> GHMRQSTLHTRLSTGPGGSMRSSIEIFNIRTRKMRVVWQTPELFE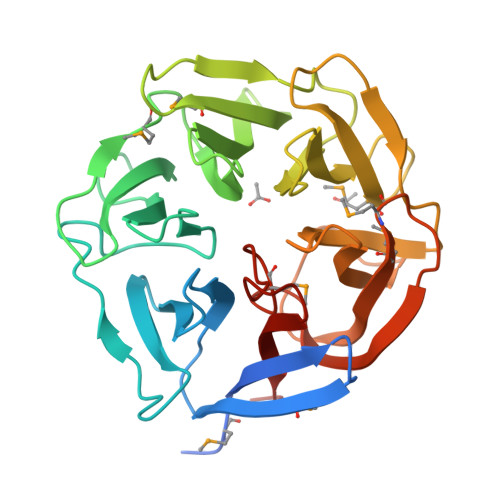APNWSPDGKYLLLNSEGLLYRLSLAGDPSPEKVDTGFATICNNDHGISPDGALYAISDKVEFGKSAIYLLPSTGGTPRLMTKNLPSYWHGWSPDGKSFTYCGIRDQVFDIYSMDIDSGVETRLTHGEGRNDGPDYSPDGRWIYFNSSRTGQMQIWRVRVDGSSVERITDSAYGDWFPHPSPSGDKVVFVSYDADVFDHPRDLDVRVQLMDMDGGNVETLFDLFGGQGTMNSPNWSPDGDEFAYVRYFPVEGS>[6x]ADIQSFSFKNFNSSSFILQGDATVSSSKLRLTKVKGNGLPTLSSLGRAFYSSPIQIYDKSTGAVASWATSFT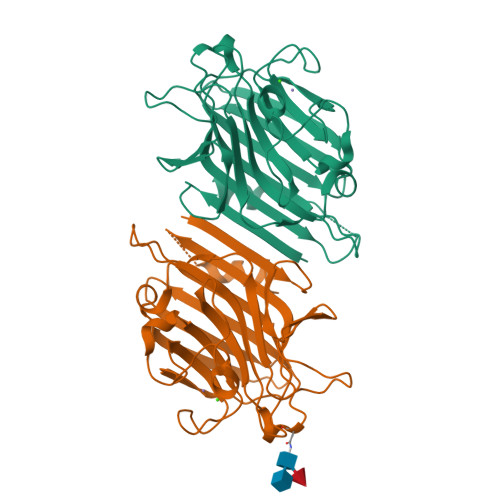ANIFAPNKSSSADGIAFALVPVGSEPKSNSGFLGVFDSDVYDNSAQTVAVEFDTFSNTDWDPTSRHIGIDVNSIKSIRTASWGLANGQNAEILITYNAATSLLVASLVHPSRRTSYIVSERVDITNELPEYVSIGFSATTGLSEGYTETHDVLSWSFASKLPDDSTTEPLDIASYLVRNVL> GSH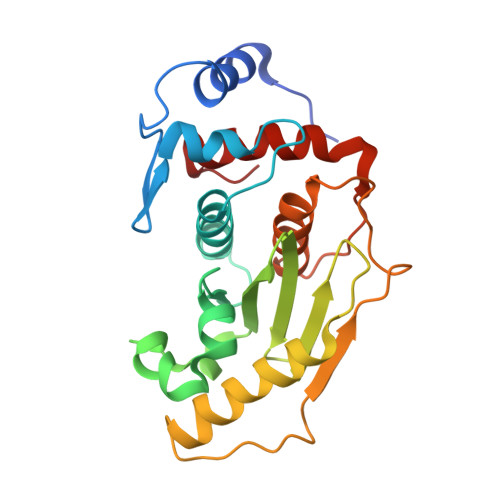MASDLLELTEDMEKEISNALGHGPQDEILSSAFKLRITRGDIQTLKNYHWLNDEVINFYMNLLVERNKKQGYPALHVFSTFFYPKLKSGGYQAVKRWTKGVNLFEQEIILVPIHRKVHWSLVVIDLRKKCLKYLDSMGQKGHRICEILLQYLQDESKTKRNSDLNLLEWTHHSMKPHEIPQQLNGSDSGMFTCKYADYISRDKPITFTQHQMPLFRKKMVWEILHQQLL> MLNKSFVKKLDESLNRKQVGSTNVTRYKIEDSYLVLAAVRVGIGGLTYHNGAAAFLEALKFWRYGENIYNLFFQRGAILNAYTTLEFTDYVFLSKEESINENLNLLLTFLYHHQYDEKTISLERNIIINEINGAGTARLNGQESIEKERHCILGSAESISRMGRKEFELISQKYYTPENTSIYVIGGNQDIDLFHIPTAVMTTQYGKPTHKVNVNEVEMNKDMILLPVEHGDYLKNRMICHLIADMIKHLAQQLEYDVSVGLFISTNQHSCYLKVKKSDQKRFSSLIQQLSMDEHFIETYIKDYQWRFMNELVINFNQLHNIYDY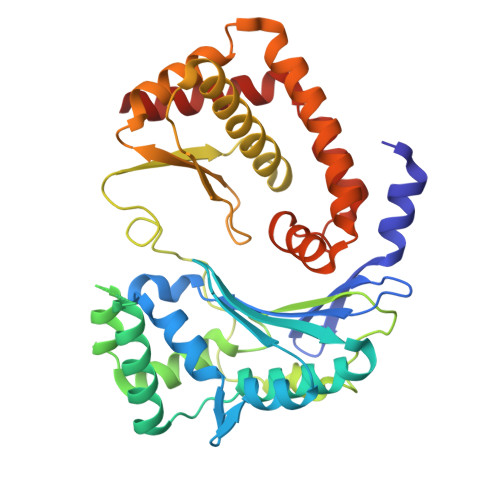MTEYRLGEYTVAELFGSLDSVDKLDILAVRNELINQLTVGE>[4x]TLVKDILSKPPITAHSNISI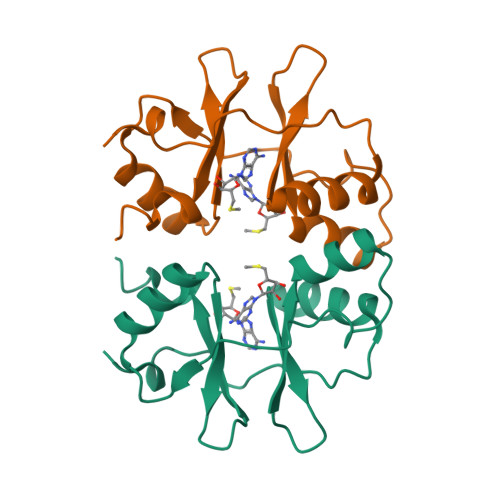MEAAKILIKHNINHLPIVDEHGKLVGIITSWDIAKALAQNKKTIEEIMTRNVITAHEDEPVDHVAIKMSKYNISGVPVVDDYRRVVGIVTSEDISRLFGGKK> AQLRQFYVAAQGISWSYRPEPTNSSLNLSVTSFKKIVYREYEPYFKKEKPQSTISGLLGPTLYAEVGDIIKVHFKNKADKPLSIHPQGIRYSKLSEGASYLDHTFPAEKMDDAVAPGREYTYEWSISEDSGPTHDDPPCLTHIYYSHENLIEDFNSGLIGPLLICKKGTLTEGGTQKTFDKQIVLLFAVFDESKSWSQSSSLMYTVNGYVNGTMPDITVCAHDHISWHLLGMSSGPELFSIHFNGQVLEQNHHKVSAITLVSATSTTANMTVGPEGKWIISSLTPKHLQAGMQAYIDIKNCPKKTRNLKKITREQRRHMKRWEYFIAAEEVIWDYAPVIPANMDKKYRSQHLDNFSNQIGKHYKKVMYTQYEDESFTKHTVNPNMKEDGILGPIIRAQVRDTLKIVFKNMASRPYSIYPHGVTFSPYEDEVNSSFTSGRNNTMIRAVQPGETYTYKWNILEFDEPTENDAQCLTRPYYSDVDIMRDIASGLIGLLLICKSRSLDRRGIQRAADIEQQAVFAVFDENKSWYLEDNINKFCENPDEVKRDDPKFYESNIMSTINGYVPESITTLGFCFDDTVQWHFCSVGTQNEILTIHFTGHSFIYGKRHEDTLT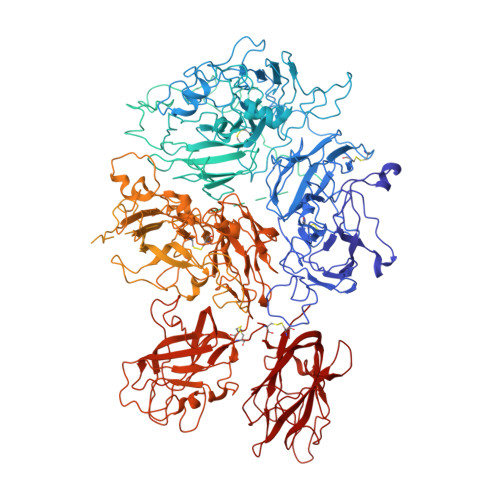LFPMRGESVTVTMDNVGTWMLTSMNSSPRSKKLRLKFRDVKCIPDDDEDSYEIFEPPESTVMATRKMHDRLEPEDEESDADYDYQNRLAAALGIRSFRNSSLNQEEEEFNLTALALENGTEFVSSNTDIIVGSNYSSPSNISKFTVNNLAEPQKAPSHQQATTAGSPLRHLIGKNSVLNSSTAEHSSPYSEDPIEDPLQPDVTGIRLLSLGAGEFKSQEHAKHKGPKVERDQAAKHRFSWMKLLAHKVGRHLSQDTGSPSGMRPWEDLPSQDTGSPSRMRPWKDPPSDLLLLKQSNSSKILVGRWHLASEKGSYEIIQDTDEDTAVNNWLISPQNASRAWGESTPLANKPGKQSGHPKFPRVRHKSLQVRQDGGKSRLKKSQFLIKTRKKKKEKHTHHAPLSPRTFHPLRSEAYNTFSERRLKHSLVLHKSNETSLPTDLNQTLPSMDFGWIASLPDHNQNSSNDTGQASCPPGLYQTVPPEEHYQTFPIQDPDQMHSTSDPSHRSSSPELSEMLEYDRSHKSFPTDISQMSPSSEHEVWQTVISPDLSQVTLSPELSQTNLSPDLSHTTLSPELIQRNLSPALGQMPISPDLSHTTLSPDLSHTTLSLDLSQTNLSPELSQTNLSPALGQMPLSPDLSHTTLSLDFSQTNLSPELSHMTLSPELSQTNLSPALGQMPISPDLSHTTLSLDFSQTNLSPELSQTNLSPALGQMPLSPDPSHTTLSLDLSQTNLSPELSQTNLSPDLSEMPLFADLSQIPLTPDLDQMTLSPDLGETDLSPNFGQMSLSPDLSQVTLSPDISDTTLLPDLSQISPPPDLDQIFYPSESSQSLLLQEFNESFPYPDLGQMPSPSSPTLNDTFLSKEFNPLVIVGLSKDGTDYIEIIPKEEVQSSEDDYAEIDYVPYDDPYKTDVRTNINSSRDPDNIAAWYLRSNNGNRRNYYIAAEEISWDYSEFVQRETDIEDSDDIPEDTTYKKVVFRKYLDSTFTKRDPRGEYEEHLGILGPIIRAEVDDVIQVRFKNLASRPYSLHAHGLSYEKSSEGKTYEDDSPEWFKEDNAVQPNSSYTYVWHATERSGPESPGSACRAWAYYSAVNPEKDIHSGLIGPLLICQKGILHKDSNMPMDMREFVLLFMTFDEKKSWYYEKKSRSSWRLTSSEMKKSHEFHAINGMIYSLPGLKMYEQEWVRLHLLNIGGSQDIHVVHFHGQTLLENGNKQHQLGVWPLLPGSFKTLEMKASKPGWWLLNTEVGENQRAGMQTPFLIMDRDCRMPMGLSTGIISDSQIKASEFLGYWEPRLARLNNGGSYNAWSVEKLAAEFASKPWIQVDMQKEVIITGIQTQGAKHYLKSCYTTEFYVAYSSNQINWQIFKGNSTRNVMYFNGNSDASTIKENQFDPPIVARYIRISPTRAYNRPTLRLELQGCEVNGCSTPLGMENGKIENKQITASSFKKSWWGDYWEPFRARLNAQGRVNAWQAKANNNKQWLEIDLLKIKKITAIITQGCKSLSSEMYVKSYTIHYSEQGVEWKPYRLKSSMVDKIFEGNTNTKGHVKNFFNPPIISRFIRVIPKTWNQSIALRLELFGCDIY>[2x]MVSVSEIRKAQRAEGPATILAIGTANPANCVEQSTYPDFYFKI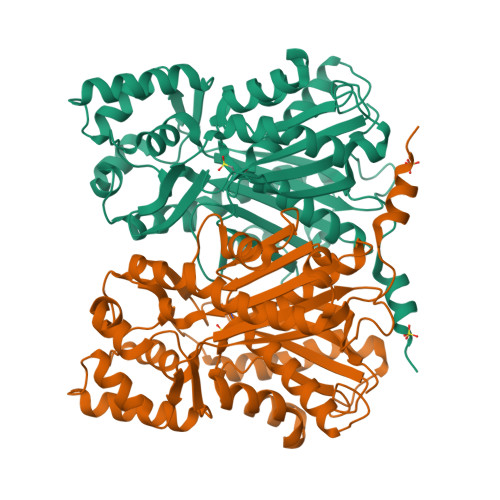TNSEHKTELKEKFQRMCDKSMIKRRYMYLTEEILKENPNVCEYMAPSLDARQDMVVVEVPRLGKEAAVKAIKEWGQPKSKITHLIVCTTSGVDMPGADYQLTKLLGLRPYVKRYMMYQQGCFAGGTVLRLAKDLAENNKGARVLVVCSEVTAVTFRGPSDTHLDSLVGQALFGDGAAALIVGSDPVPEIEKPIFEMVWTAQTIAPDSEGAIDVHLREAGLTFHLLKDVPGIVSKNITKALVEAFEPLGISDYNSIFWIAHPGGPAILDQVEQKLALKPEKMNATREVLSEYGNMSSACVLFILDEMRKKSTQNGLKTTGEGLEWGVLFGFGPGLTIETVVLRSVAI> ADGPYLVIVEQPKQRGFRFRYGCEGPSHGGLPGASSEKGRKTYPTVKICNYEGPAKIEVDLVTHSDPPRAHAH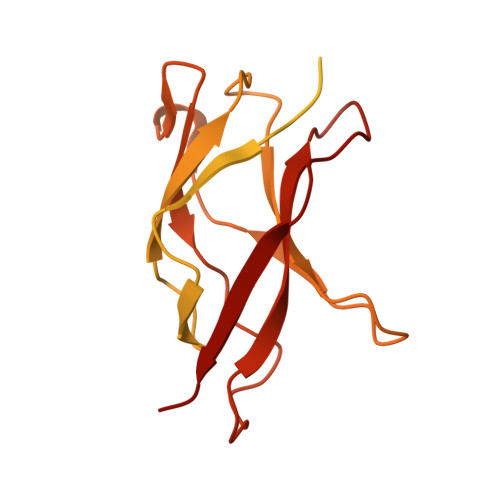SLVGKQCSELGICAVSVGPKDMTAQFNNLGVLHVTKKNMMGTMIQKLQRQRLRSRPQGLTEAEQRELEQEAKELKKVMDLSIVRLRFSAFLRASDGSFSLPLKPVISQPIHDSKSPGASNLKISRMDKTAGSVRGGDEVYLLCDKVQKDDIEVRFYEDDENGWQAFGDFSPTDVHKQYAIVFRTPPYHKMKIERPVTVFLQLKRKRGGDVSDSKQFTYYPLV> MGSSHHHHHHSSGHMFKYEDIPADYRDLMPPEARDFLQNLSDGDKTVLKEVFKAGPYKNTEESIAALKKKSPELGAKVEKLHAMVKSKIAALGPEAKGFAEKSIEIARGIKARYYTGNEPTKDDLKASVKEVLKLYKAMSDAGKADFGKQFPFLAKVFESGKAAKFAGEN

Fatty acid and retinol-binding proteins (FARs) comprise a family of unusual α-helix rich lipid-binding proteins found exclusively in nematodes. They are secreted into host tissues by parasites of plants, animals and humans. The protein Na-FAR-1 derives from the blood feeding intestinal hookworm of humans, N. americanus. The 3D structure of Na-FAR-1 in its ligand-free and ligand-bound forms, determined by NMR (nuclear magnetic resonance) spectroscopy and X-ray crystallography respectively, reveals an α-helical fold similar to Ce-FAR-7, but Na-FAR-1 possesses a larger and more complex internal ligand-binding cavity and an additional C-terminal α-helix.

Na-FAR-1, which had not been subjected to reverse phase HPLC purification to strip out co-purifying ligands, crystallized as previously reported and diffracted to 2.14 Å. Molecular replacement using the Ce-FAR-7 structure proved unsuccessful and we therefore obtained the crystal structure of Na-FAR-1 in complex with co-purifying ligands, hereafter referred to as holo-Na-FAR-1, by anomalous dispersion from crystals of Se-Met-labelled protein. Na-FAR-1 presents a wedge-shaped structure with two larger faces each of approximately 40 by 30 Å in area and of ∼17 Å in width at the wide end of the wedge. The fold is organized into 11 helices of various lengths, defining an internal cavity. The internal cavity is much larger for the holo protein, achieved by a global outward displacement of the surrounding helices by a little over 1 Å compared with the apo form, with the biggest changes seen at the C-terminal end of helix α7. In the holo form, the cavity is more than twice as big, reaching 2570 and 2170 Å3 for probes of 1.4 and 1.925 Å respectively. In the holo structure the expanded cavity is lined by the same residues as in the apo structure, but with 21 additional, predominantly apolar, side chains contributing to the surface of the expanded cavity (Phe1, Ile6, Leu25, Lys30, Lys34, Val36, Ser48, Ile49, Leu52, Met69, Phe84, Ala85, Ile91, Ile95, Tyr99, Leu110, Ser113, Phe132, Phe136, Val142 and Ala148). In addition to the opening seen in the apo form, the cavity is also accessible to solvent via an opening between the α2–α3 and α9–α10 turns and α6. Within the cavity of the holo form, clear electron density was observed that is well fitted by a single FA molecule, containing 16 carbon atoms. The palmitate appears to be curled into a C-shape around the side chain of Lys96 and contacts 11 other residues (Phe1, Ile6, Met14, Phe21, Leu22, Leu25, Leu33, Leu66, Ile95, Tyr99 and Tyr100).> QDNSRYTHF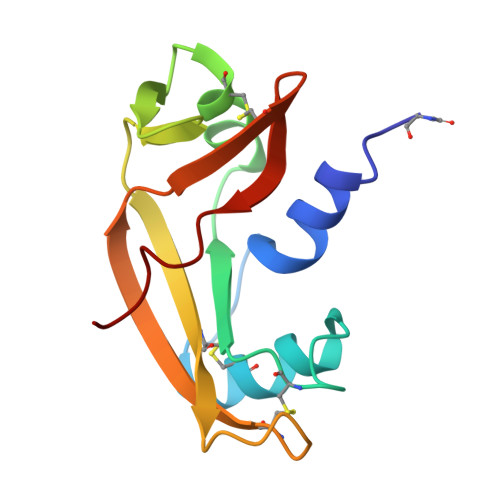LTQHYDAKPQGRDDRYCESIMRRRGLTSPCKDINTFIHGNKRSIKAICENKNGNPHRENLRISKSSFQVTTCKLHGGSPWPPCQYRATAGFRNVVVACENGLPVHLHQSIFRRP>MPLGLLWLGLALLGALHAQAQDSTSDLIPAPPLSKVPLQQNFQDNQFQGKWYVVGLAGNAILREDKDPQKMYATIYELKEDKSYNVTSVLFRKKKCDYWIRTFVPGSQPGEFTLGNIKSYPGLTSYLVRVVSTNYNQHAMVFFKAVSQNREYFAITLYGRTKELTSELKENFI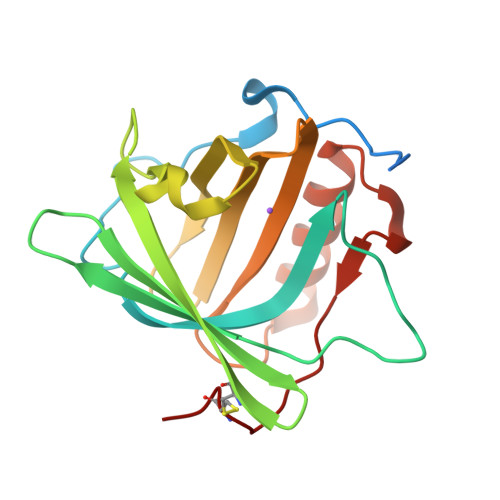RFSKSLGLPENHIVFPVPIDQCIDG[3x]>[2x]SDERHKTDIAPISDKVLDAWEKVKFYQYKFKDAVDEKGEEARYHFGVIAQQIVKVFEDEGLSAFDYGLVGYDEWEATEDEYDSEGNLVEKGREAGNIYSIRPTECQWLE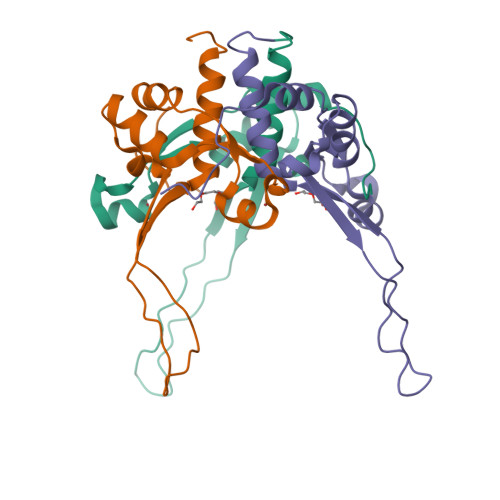MACMRRKLERLSLEHHHHHH3-[(3~{a}~{S},4~{R},8~{a}~{S},8~{b}~{R})-4-[5-(5-chloranylthiophen-2-yl)-1,2-oxazol-3-yl]-1,3-bis(oxidanylidene)-4,6,7,8,8~{a},8~{b}-hexahydro-3~{a}~{H}-pyrrolo[3,4-a]pyrrolizin-2-yl]propyl-trimethyl-azanium 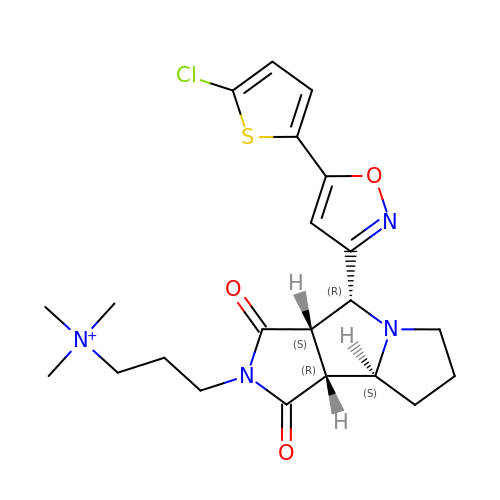| C22 H28 Cl N4 O3 S | IMQAZTOPHVBANA-DSYPUSFNSA-N E. coli tryptophanase (tryptophan indole-lyase, Trpase, EC 4.1.99.1) is a pyridoxal 5'-phosphate (PLP)-dependent enzyme that catalyses α,β-elimination and β-replacement reactions of L-tryptophan. Trpase consists of four identical subunits (~52 kD per monomer), each of which covalently binds one molecule of PLP. The tetramer possesses a D2 symmetry, therefore it is a dimer of dimers with two different dimeric interfaces: a catalytic interface and a non-catalytic interface. Using kinetic spectrophotometric methods and size-exclusion chromatography we have previously shown that the inactivation process is linked to the cleavage of the PLP-Lys270 aldimine bond and to the dissociation of the tetrameric form of Trpase into dimers.

The two apo mutants of E. coli Trpases as well as the wt Trpase are found in an open conformation, different than that of the closed one found for P. vulgaris in its holo form. The RMS deviation for 464 Cás of the C298S mutant crystal structure with the Trpase from P. vulgaris (of subunit A) is 4.8 Å, while the RMS deviation for each domain is 2.1 Å for the large domain (for 260 Cαs) and 1.1 Å for the small domain (for 152 Cαs of the small domain). Residue 330 of E. coli Trpase is located at the non-catalytic interface while residue 298 is located at the catalytic interface, yet both mutants showed a similar loss of activity. The rate constants of the initial linear phase are (13.8 ± 0.3) × 10-3 min-1, (1.7 ± 0.1) × 10-3 min-1 and (0.6 ± 0.3) × 10-3 min-1 for C298S, W330F and wt Trpase, respectively. Both W330F and C298S exhibit similar (90%) total cold inactivation, but the time profile revealed a factor of about 8 fold faster kinetics for C298S. The rate constants for cold inactivation and dissociation are similar for the wt and the W330F mutant, but in the case of C298S there is a factor of ~4 between them. This may be attributed to the relative proximity of residue 298 to the PLP and substrate binding sites as well as to its location on the catalytic interface, in contrast to that of the 330 site. The PLP in the C298S mutant is loosely bound allowing, relative to W330F and the wt, a quicker cold inactivation and dissociation. In one of the wt apo crystal structures this loop is found in the same conformation as holo P. vulgaris Trpase. This suggests that the loop composed of residues 295-310 is highly flexible and may be involved in the transition between the closed and open conformation. The flexibility of this region may account for the faster kinetics found for C298S mutant. The location of the point mutation, i.e. on the catalytic (C298S) vs. the non-catalytic (W330F) axis, affects primarily the kinetics of cold lability.

> KHLPEPFRIRVIEPVKRTTRAYREEAIIKSGMNPFLLDSEDVFIDLLTDSGTGAVTQSMQAAMMRGDEAYSGSRSYYALAESVKNIFGYQYTIPTHQGRGAEQIYIPVLIKKREQEKGLDRSKMVAFSNYFFDTTQGHSQINGCTVRNVYIKEAFDTGVRYDFKGNFDLEGLERGIEEVGPNNVPYIVATITSNSAGGQPVSLANLKAMYSIAKKYDIPVVMDSARFAENAYFIKQREAEYKDWTIEQITRETYKYADMLAMSAKKDAMVPMGGLLCMKDDSFFDVYTECRTLSVVQEGFPTYGGLEGGAMERLAVGLYDGMNLDWLAYRIAQVQYLVDGLEEIGVVCQQAGGHAAFVDAGKLLPHIPADQFPAQALACELYKVAGIRAVEIGSFLLGRDPKTGKQLPCPAELLRLTIPRATYTQTHMDFIIEAFKHVKENAANIKGLTFTYEPKVLRHFTAKLKEV> MNRWVEKWLRVYLKCYINLILFYRNVYPPQ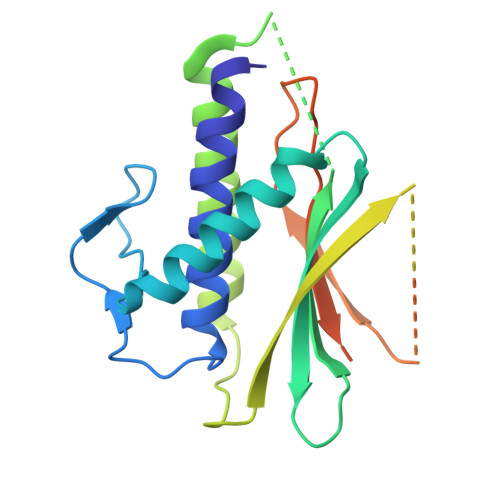SFDYTTYQSFNLPQFVPINRHPALIDYIEELILDVLSKLTHVYRFSICIINKKNDLCIEKYVLDFSELQHVDKDDQIITETEVFDEFRSSLNSLIMHLEKLPKVNDDTITFEAVINAIELELGHKLDRNRRVDSLEEKAEIERDSNWVKCQEDENLPDNNGFQPPKIKLTSLVGSDVGPLIIHQFSEKLISGDDKILNGVYSQYEEGESIFGSLF>[4x]MVPTQAHPEWYKSAVFYELSVRTFQDGNGDGKGDFPGLTSRLDYLKNLGVDCLWLLPWFPSPLRDDGYDVADYRGIHPDLGTLDDFKVFLREAHARGLWVIGDLVTNHTSSDHPWFQAARRGPTLPDGSPNEYHDYYVWSDEGKEYADTRIIFTDTEVSNWTLDEQAGKYYWHRFFASQPDLNYDNPKVVEELHGAARFWLDLGLDGFRVDAVPYLIEREGTSCENLPETHEILKGFRAMVDREYPGRLLLAEAAQWPEEVVEYFGTEAEPEFHMCFNFPVMPRLYMSLKREDTSSIREIMGRLPKIPSFGQWCIFLRNHDELTLEMVTDDERAFMYAAYAPDARMKINVGIRRRLAPLLDNDRRRIELLNTVLLALPGSPVLYYGDEIGMGDDLGLPDRNGVRTPMQWNAGTSGGFSTAQPSDCFFPPIQDPVYGFGRVNVQSQLQDPSSLLKWTAR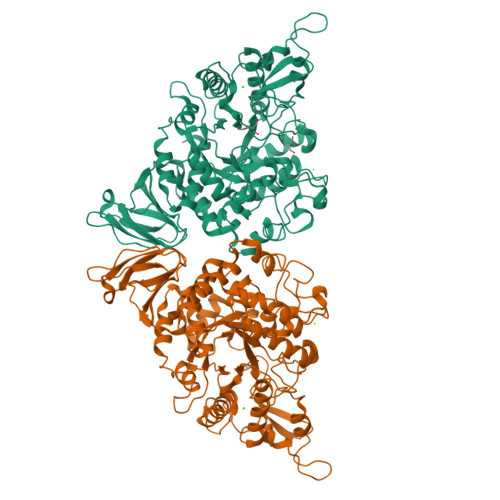QLELRRAHPAFAHGDLTFIETGNPAILAFTRQYDGETLLIVSNFAGNAQAGLLDLAPFVGRAPVTLSGASPLPVVTGNGQYPVVMGKYDYYWLRLNSRVDKLAAALEHHHHHH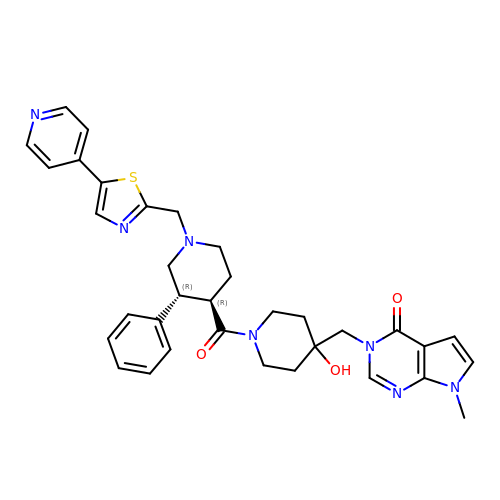7-methyl-3-[[4-oxidanyl-1-[(3~{R},4~{R})-3-phenyl-1-[(5-pyridin-4-yl-1,3-thiazol-2-yl)methyl]piperidin-4-yl]carbonyl-piperidin-4-yl]methyl]pyrrolo[2,3-d]pyrimidin-4-one | C34 H37 N7 O3 S | RRXAAUXUWASHNO-IAPPQJPRSA-N> GGAUCCCGACUGGCGAGAGC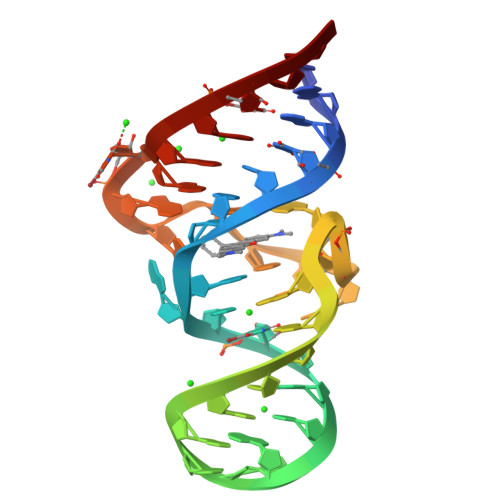CAGGUAACGAAUGGAUCC> SLNDKPVGFASVPTADLPEGTVGGLGGEIVFVRTAEELEKYTTAEGKYVIVVDGTIVFEPKREIKVLSDKTIVGINDAKIVGGGLVIKDAQNVIIRNIHFEGFYMEDD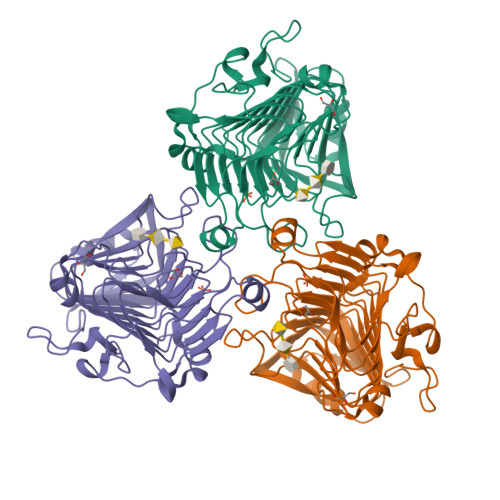PRGKKYDFDYINVENSHHIWIDHITFVNGNDGAVDIKKYSNYITVSWNKFVDHDKVSLVGSSDKEDPEQAGQAYKVTYHHNYFKNLIQRMPRIRFGMAHVFNNFYSMGLRTGVSGNVFPIYGVASAMGAKVHVEGNYFMGYGAVMAEAGIAFLPTRIMGPVEGYLTLGEGDAKNEFYYCKEPEVRPVEEGKPALDPREYYDYTLDPVQDVPKIVVDGAGAGKLVFEELNTAQ> MEEREERVRDDTIEEFATYLELEGKSRNTVRMYTYYISKFFEEGHSPTARDALRFLAKLKRKGYSTRSLNLVIQALKAYFKFEGLDSEAEKLKTPKMPKTLPKSLTEEEVRRIINAAETLRDRLILLLLYGAGLRVSELCNLRVEDVNFEYGVIVVRGGKGGKDRVVPISESLLSEIKRYLESRNDDSPYLFVEMKRKR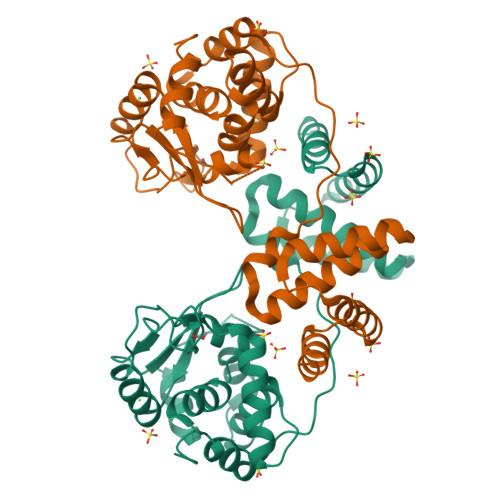KDKLSPKTVWRLVKKYGRKAGVELTPHQLRHSFATHMLERGIDIRIIQELLGHSNLSTTQIYTKVSTKHLKEAVKKAKLVESIIGGSHHHHHH buta-2,3-dien-1-yl trihydrogen diphosphate | C4 H8 O7 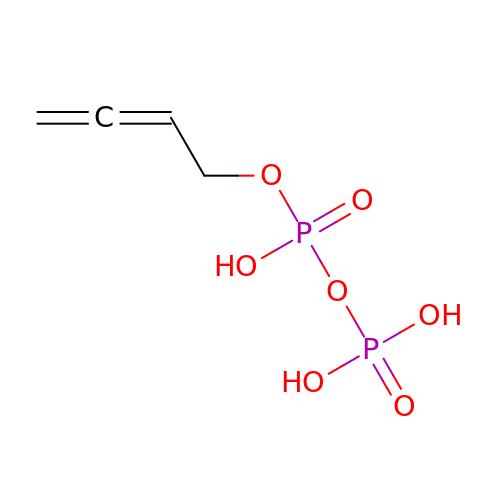P2 | SBJIRHJBHHXSDO-UHFFFAOYSA-N4-PHENYLBUTYLAMINE 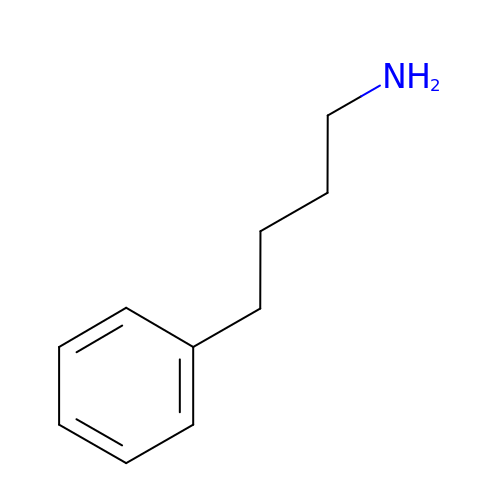| C10 H15 N | AGNFWIZBEATIAK-UHFFFAOYSA-N>PPGP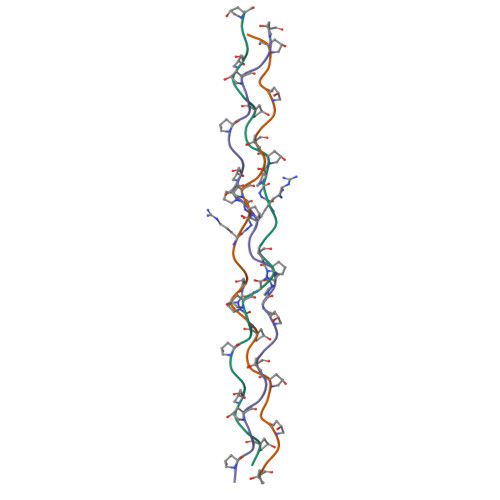PGPPGPPGXPGPRXPPGPPGPPGPPG[6x]>[2x]SNAYRGPEAFLK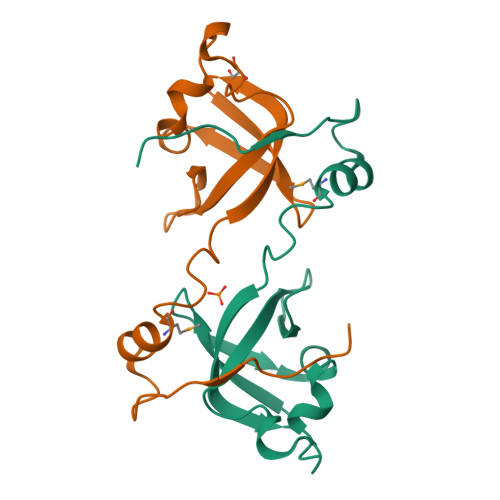LPKDLKDREALQDIMQDIGNSDDILAAVVLSATPGAVEAFRKNGETIRITGDGLKAAHRFLSNDPKIGEKRIRPGALIRVKKTEKGSWQIVQLP>[8x]GSMQNTT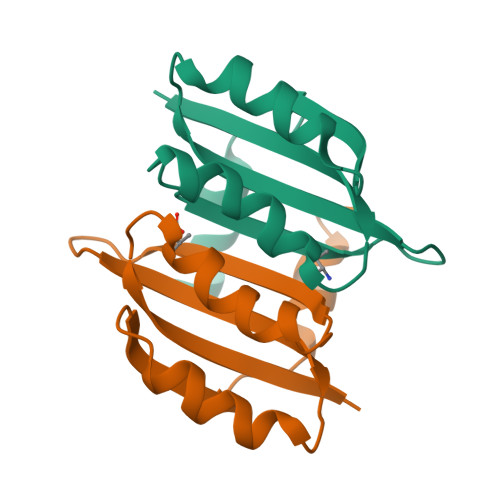HDNVILELTVRNHPGVMTHVCGLFARRAFNVEGILCLPIQDSDKSHIWLLVNDDQRLEQMISQIDKLEDVVKVQRNQSDPTMFNKIAVFFQ> MRLLYLHADRFEYKTVKPALKNPPDPPGEASFGEALVVFTTVEDGDGPQTVMYAASDIASHSSRLKVTTVILYPYAHLSSRLAKPMAAHKRLIELEGALRTKFPGHVHRAPFGWAKSFSIACKGHPLAELSRSFTE

We have been interested in a D-aminoacyl-tRNA deacylase (DTD) fold that is present across the domains of life in two different functional contexts: as an N-terminal editing domain (NTD) of archaeal ThrRS, which specifically removes non-cognate L-serine mischarged on tRNAThr, and as a freestanding ‘chiral proofreading' enzyme, which removes D-amino acids from tRNAs in bacteria and eukaryotes. Both share a striking structural and mechanistic similarity highlighting a common ancestry. Here we show, with the help of structural, biochemical and biophysical studies from three distant organisms, that the substrate specificity in this domain is determined by a differential remodelling of the catalytic centre at the RNA–protein interface rather than just the presence or absence of catalytic water as previously proposed. While demonstrating that the tRNA provides the catalytic group, we show that the side chains within the recognition site are dispensable for the proofreading function, suggesting a primordial mode of protein- or peptide scaffold-based enzymatic activity evolved alongside that of RNA.

To rule out any genus-related phenomenon and to test the universality of the observation, we chose to do biochemical experiments with NTD from Aeropyrum pernix (ApNTD), which belongs to a different phylum (Crenarchaeota), and shares ∼43% identity with PabNTD. Remarkably, the corresponding mutants Y115A, E129A and Y115A/E129A in ApNTD also retained completely the capability to discriminate between seryl and threonyl substrates. Structural studies were also carried out with the mutants of the amino-acid pocket in ApNTD. While E129A mutant also showed a loosening of interactions upon L-Thr3AA binding as observed in the case of wild type, no such loosening was observed in the case of Y115A, thus providing a rationale for rejecting the cognate substrate in the mutants.>[2x]GSHMSRVQLALRVPDLEASIGFYSKLFGTGPAKVRPGYANFAIAEPPLKLVLIEGAGEDATRLDHLGVEVEDSAQVGHAARRLKESGLA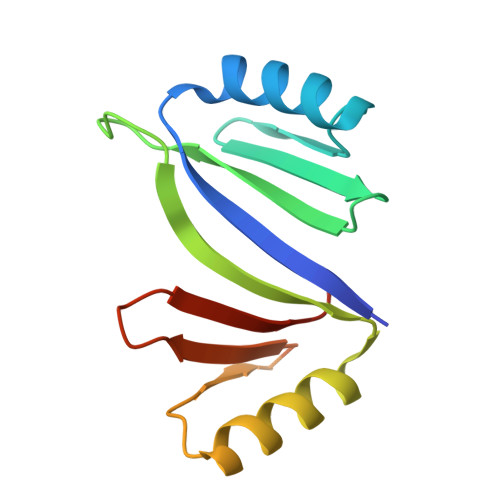TVEENDTACCYAVQDEVWVTGPGGEPWEVYVVKGDAD> MAVLEIIKHPNEVLETPCERVINFDKKLVKLLKDMHETMLIADGVGLAAPQVGVSLQVAVVDVDDDTGKIELINPSILEKRGEQVGPEGCLSFPGLYGEVERADYIKVRAQNRRGKVFLLEAEGFLARAIQH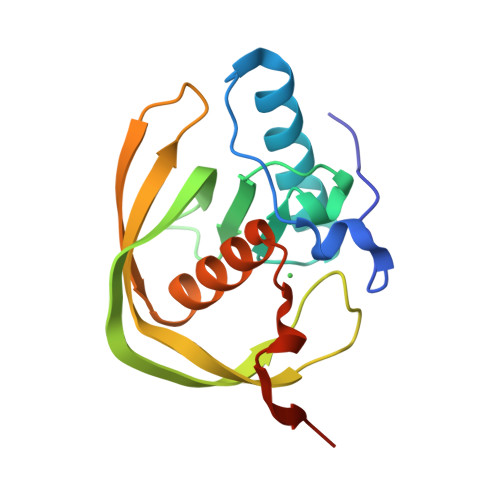EIDHLHGVLFTSKVTRYYEENELE> 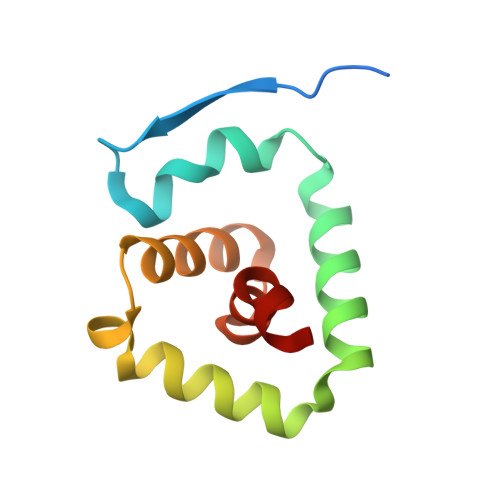DRHHHHHHGSPAPPRVNVSLDAAPAARWLPVLRLFDPGLLRAAVARIVGDRVPKWVRDVIGKLVAEMESFLPQPYTEEIRGISDFLNLSLADGFIVNLAYEASAF> ALDTTWKEATLPQVKAMLQKDTGKVSGDTVTYSGKTVHVVAAAVLPGFPFPSFEVHGKKNPTLDIPGGATVDVTFINTNKGFGHSFDITQKVPPY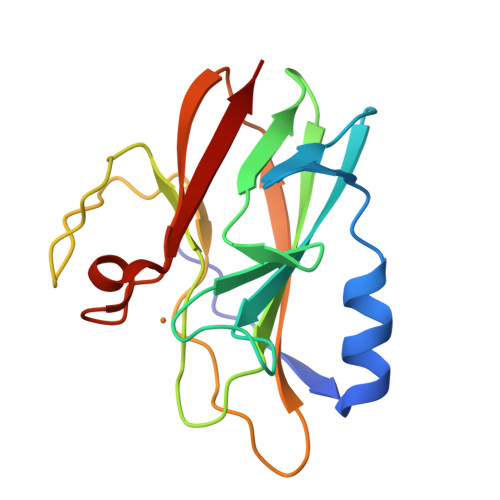AVMPVIDPIVAGTGFSPVPKDGKFGYTNFTWHPTAGTYYYVCQIPGHAATGMFGKIIVK> GPHMLEMVTDQFGMIGLLTFIRAAETDPGMVHLALGSDLTTLGLNLNSPENLYPKFASPWASSPCRPQDIDFHVPSEYLTNIHIRDKLAAIKLGRYGEDLLFYLYYMNGGDVLQLLAAVELFNRDWRYHKEERVWITRAPGMEPTMKTN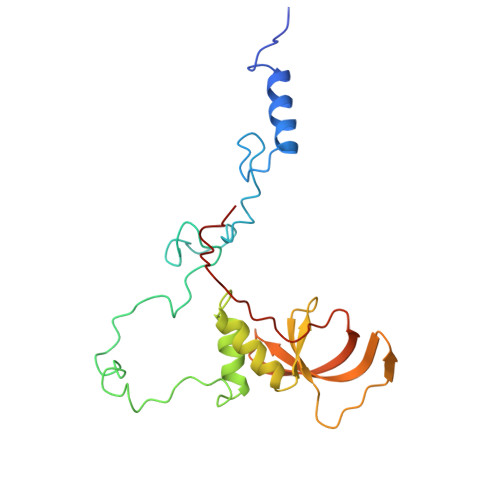TYERGTYYFFDCLNWRKVAKEFHLEYDKLEERPHLPSTFNYNPAQQAF> MSEESQAFQRQLTALIGYDVTDVSNVHDDELEFTRRGLVTPRMAEVASRDPKLYAMHPWVTSKPLPEYLWKKIANNCIFIVIHRSTTSQTIKVSPDDTPGAILQSFFTKMAKKKSLMDIPESQSEQDFVLRVCGRDEYLVGETPIKNFQWVRHCLKNGEEIHVVLDTPPDPALDEVRKEEWPLVDDCTGVTGYHEQLTIHGKDHESVFTVSLWDCDRKFRVKIRGIDIPVLPRNTDLTVFVEANIQHGQQVLCQRRTSPKPFTEEVLWNVWLEFSIKIKDLPKGALLNLQIYCGKAPALSSKASAESPSSESKGKVQLLYYVNLLLIDHRFLLRRGEYVLH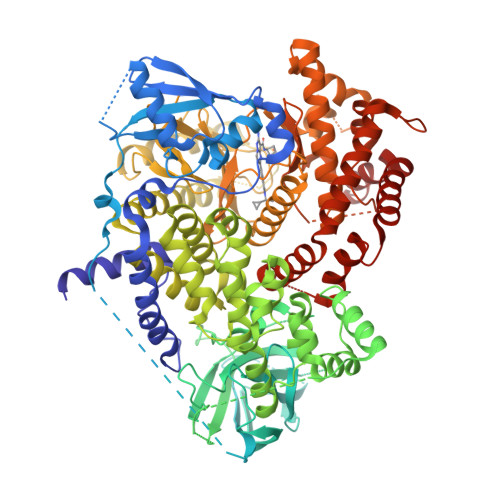MWQISGKGEDQGSFNADKLTSATNPDKENSMSISILLDNYCHPIALPKHQPTPDPEGDRVRAEMPNQLRKQLEAIIATDPLNPLTAEDKELLWHFRYESLKHPKAYPKLFSSVKWGQQEIVAKTYQLLARREVWDQSALDVGLTMQLLDCNFSDENVRAIAVQKLESLEDDDVLHYLLQLVQAVKFEPYHDSALARFLLKRGLRNKRIGHFLFWFLRSEIAQSRHYQQRFAVILEAYLRGCGTAMLHDFTQQVQVIEMLQKVTLDIKSLSAEKYDVSSQVISQLKQKLENLQNSQLPESFRVPYDPGLKAGALAIEKCKVMASKKKPLWLEFKCADPTALSNETIGIIFKHGDDLRQDMLILQILRIMESIWETESLDLCLLPYGCISTGDKIGMIEIVKDATTIAKIQQSTVGNTGAFKDEVLNHWLKEKSPTEEKFQAAVERFVYSCAGYCVATFVLGIGDRHNDNIMITETGNLFHIDFGHILGNYKSFLGINKERVPFVLTPDFLFVMGTSGKKTSPHFQKFQDICVKAYLALRHHTNLLIILFSMMLMTGMPQLTSKEDIEYIRDALTVGKNEEDAKKYFLDQIEVCRDKGWTVQFNWFLHLV> PISPIETVPVKLKPGMDGPKVKQWPLTEEKIKALVEICTEMEKEGKISKIGPENPYNTPVFAIKKKDGTKWRKLVDFRELNKKTQDFWEVQLGIPHPAGLKKKKSVTVLDVGDAYFSVPLDEDFRKYTAFTIPSINNETPGIRYQYNVLPQGWKGSPAIFQSSMTKILEPFRKQNPDIVIYQYMDDLYVGSDLEIGQHRTKIEELRQHLLRWGLTTPDKKHQKEPPFLWMGYELHPDKWTVQPIVLPEKDSWTVNDIQKLVGKLNWASQIYPGIKVRQLCKLLRGTKALTEVIPLTEEAELELAENREILKEPVHGVYYDPSKDLIAEIQKQGQGQWTYQIYQEPFKNLKTGKYARMRGAHTNDVKQL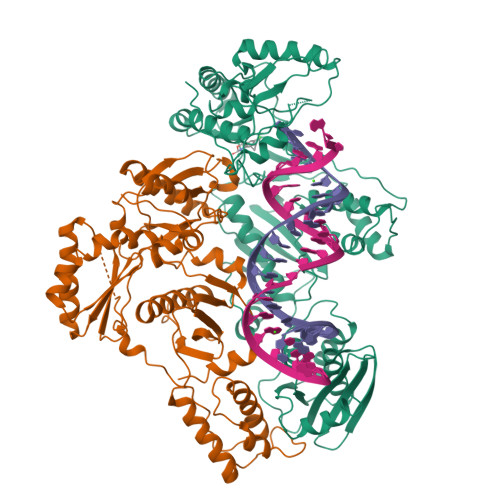TEAVQKITTESIVIWGKTPKFKLPIQKETWETWWTEYWQATWVPEWEFVNTPPLVKLWYQLEKEPIVGAETFYVDGAASRETKLGKAGYVTNKGRQKVVTLTDTTNQKTELQAIHLALQDSGLEVNIVTDSQYALGIIQAQPDQSESELVNQIIEQLIKKEKVYLAWVPAHKGIGGNEQVDKLVSAGIRKIL;> GPISPIETVPVKLKPGMDGPKVKQWPLTEEKIKALVEICTEMEKEGKISKIGPENPYNTPVFAIKKKDGTKWRKLVDFRELNKKTQDFWEVQLGIPHPAGLKKKKSVTVLDVGDAYFSVPLDEDFRKYTAFTIPSINNETPGIRYQYNVLPQGWKGSPAIFQSSMTKILEPFRKQNPDIVIYQYMDDLYVGSDLEIGQHRTKIEELRQHLLRWGLTTPDKKHQKEPPFLWMGYELHPDKWTVQPIVLPEKDSWTVNDIQKLVGKLNWASQIYPGIKVRQLCKLLRGTKALTEVIPLTEEAELELAENREILKEPVHGVYYDPSKDLIAEIQKQGQGQWTYQIYQEPFKNLKTGKYARMRGAHTNDVKQLTEAVQKITTESIVIWGKTPKFKLPIQKETWETWWTEYWQATWVPEWEFVNTPPLVKLWYQLEKEPIVGAETF> CFAKGTNVLMADGSIECIENIEVGNKVMGKDGRPREVIKLPRGRETMYSVVQKSQHRAHKSDSSREVPELLKFTCNATHELVVRTPRSVRRLSRTIKGVEYFEVITFEMGQ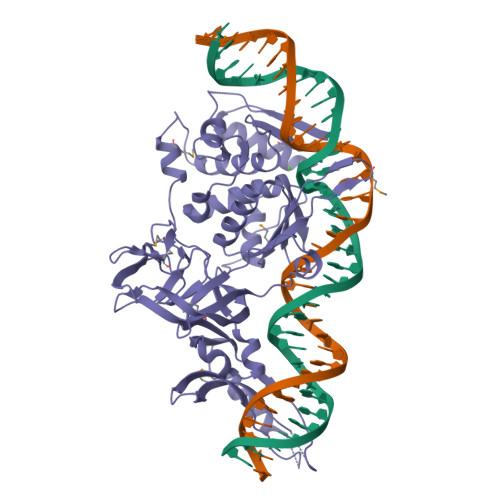KKAPDGRIVELVKEVSKSYPISEGPERANELVESYRKASNKAYFEWTIEARDLSLLGSHVRKATYQTYAPILYENDHFFDYMQKSKFHLTIEGPKVLAYLLGLWIGDGLSDRATFSVDSRDTSLMERVTEYAEKLNLCAEYKDRKEPQVAKTVNLYSKVVRGNGIRNNLNTENPLWDAIVGLGFLKDGVKNIPSFLSTDNIGTRETFLAGLIDSDGYVTDEHGIKATIKTIHTSVRDGLVSLARSLGLVVSVNAEPAKVDMNGTKHKISYAIYMSGGDVLLNVLSKCAGSKKFRPAPAAAFARECRGFYFELQELKEDDYYGITLSDDSDHQFLLANQVVVHN> SEAEARPTNFIRQIIDEDLASGKHTTVHTRFPPEPNGYLHIGHAKSICLNFGIAQDYKGQCNLRFDDTNPVKEDIEYVESIKNDVEWLGFHWSGNVRYSSDYFDQLHA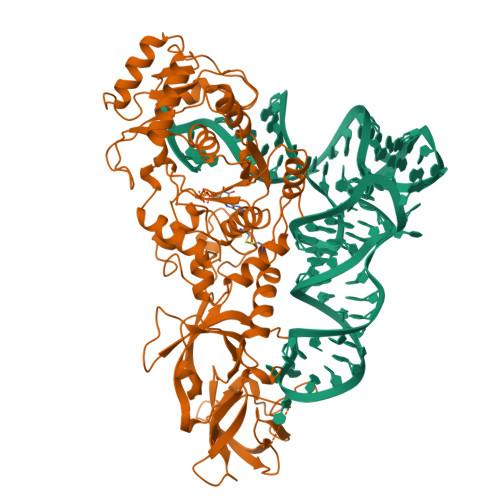YAIELINKGLAYVDELTPEQIREYRGTLTQPGKNSPYRDRSVEENLALFEKMRAGGFEEGKACLRAKIDMASPFIVMRDPVLYRIKFAEHHQTGNKWCIYPMYDFTHCISDALEGITHSLCTLEFQNNRRLYDWVLDNITIPVHPRQYEFSRLNLEYTVMSKRKLNLLVTDKHVEGWDDPRMPTISGLRRRGYTAASIREFCKRIGVTKQDNTIEMASLESCIREDLNENAPRAMAVIDPVKLVIENYQGEGEMVTMPNHPNKPEMGSRQVPFSGEIWIDRADFREEANKQYKRLVLGKEVRLRNAYVIKAERVEKDAEGNITTIFCTYDADTLSKDPADGRKVKGVIHWVSAAHALPVEIRLYDRLFSVPNPGAADDFLSVINPESLVIKQGFAEPSLKDAVAGKAFQFEREGYFCLDSRHSTAEKPVFNRTVGLRDTWAKVGE>GSHMPKRTFTKEDIRKFAEEENVRYLRLQFTDILGTIKNVEVPVSQLEKVLDNEMMFDGSSIEGFVRIEESDMYLHPDLDTWVIFPWTAGQGKVARLICD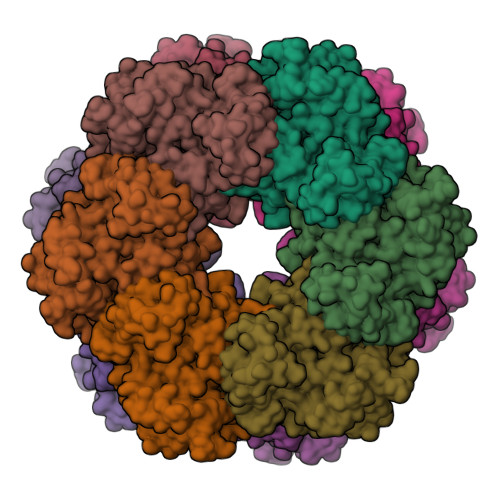VYKTDGTPFEGDPRANLKRVLKEMEDLGFTDFNLGPEPEFFLFKLDEKGEPTLELNDDGGYFDLAPTDLGENCRRDIVLELEDMGFDIEASHHEVAPGQHEIDFKYADAVTACDNIQTFKLVVKTIARKHNLHATFMPKPLFGVNGSGMHFNVSLFKGKENAFFDPNTEMGLTETAYQFTAGVLKNARGFTAVCNPLVNSYKRLVPGYEAPCYIAWSGKNRSPLIRVPSSRGLSTRIEVRSVDPAANPYMALAAILEAGLDGIKNKLKVPEPVNQNIYEMNREEREAVGIQDLPSTLYTALKAMRENEVIKKALGNHIYNQFINSKSIEWDYYRTQVSEWERDQYMKQY[12x];>[12x]PINRGDLSRFI>SEHKAKYENVTKDIFDLRDYYSGASKELKNVTGYRYSKGGKHYLIFDKHQKFTRIQIFGKDIERLKTRKNPGLDIFVVKEAENRNGTVFSYGGVTKKNQGAYYDYLNAPKFVIKKEVDAGVYTHVKRHYIYKEEVSLKE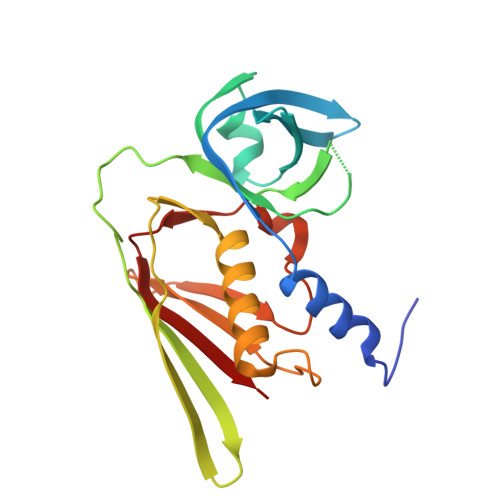LDFKLRQYLIQNFDLYKKFPKDSKIKVIMKDGGYYTFELNKKLQPHRMSDVIDGRNIEKMEANIR[2x]>[2x]HMMAGNDSNLIWLDLEMTGLEPVEDVILEIAIIITDSELNILAQGPIFAISQTDDVLDNMNPWCIEHHGKSGLTQRCRDSEVSLAHATKESLAFVQEWVPQGKSPMCGNSIGQDRRFINKYMPDFEDHFHYRNLDVSTIKELAKRWKPEVLESVVKTGAHLALDDIKESIAELKVYRELFFKL

Therefore, oligoribonucleases (ORN), RNases targeted toward short oligonucleotides, are needed for the complete digestion of short oligonucleotides into mononucleotides. Among these, ORN belongs to the DEDD superfamily, comprising 3′-5′ exonucleases that require a divalent cation for activity. Our research group have focused on the mechanism of action of oligoribonuclease (CpsORN) from the psychrophilic gram-negative bacterium Colwellia psychrerythraea strain 34H, to understand how the enzyme hydrolyses small nucleic acids. Structural analysis results show that CpsORN is a stable dimer and its active site is formed by swapping residues from the other subunit.

We also report the structure of two separate uridine-bound forms that mimic the product bound state of CpsORN. Furthermore, the structure of CpsORN bound to two separated uridines was determined to understand how the cleaved products interact with CpsORN. In this structure, two uridine mononucleotides are located in similar positions as the last two 3′-terminal nucleotides of the U-U complex structure. Both uridine molecules interact with the manganese ion. The O atom from the phosphate of U2 directly interacts with manganese, and the C3 atom of U1 is located near the manganese ion and the O atom of U2. Structural comparison between separated uridine-bound structure and unliganded-structure clearly shows a prominent difference in their flexible loop region. The His158 residue showed inward movement toward the active site to interact with the cleaved uridine phosphate, in the two-uridine complex structure. Thus, the His158 was suspected as an activator of the water molecule during the enzymatic reaction of CpsORN. In separated two-uridine-bound structure, manganese ion has a different interaction network compared with those of the U-U complex structure. In particular, the manganese ion forms a new interaction with the 3′-oxygen of the ribose in the U1 ribonucleotide.>LSRLALEADLRGAIGRGEITPYFQPIVRLSTGALSGFEALARWIHPRRGMLPPDEFLPLIEEMGLMSELGAHMMHAAAQQLSTWRAAHPAMGNLTVSVNLSTGEIDRPGLVADVAETLRVNRLPRGALKLEVTESDIMRDPERAAVILKTLRDAGAGLA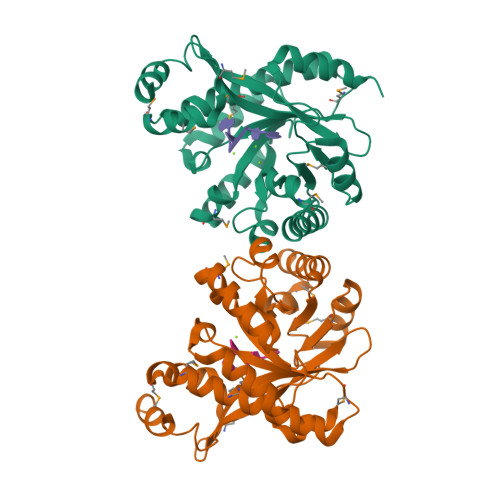LDDFGTGFSSLSYLTRLPFDTLKIDRYFVRTMGNNAGSAKIVRSVVKLGQDLDLEVVAEGVENAEMAHALQSLGCDYGQGFGYAPALSPQEAEVYLNEAYVD[2x]>MSNAEKALGVALIGTGFMGKCHAMAWRNVATAFGGLPPRLEVLADMPADKAHSLASSFGFARGTADWREAVSDPAVDVVSITTPNGLHREMAEAALAAGKHVWLEKPMALSVEDAQAMEAAARASDRRTIIGYNYTRSPAFRAAVDLIAEGAIGRPIHFRGMYDEDYMADPDLPWSWALTRKDGGLGALGDLGCHLVSVMVSLMGPVARVYAQADTVITDRPHQGGTARVENEDQAQALIRFASGTSGEFSCSRVARGYRCRLAWEVQGTEGTLRFDQERMNE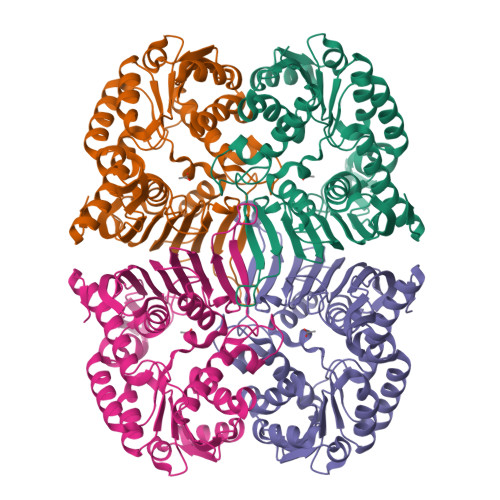LWLYQPGRPEIDGFRRILTGPAQPGFAAFCPGGGHNFGFNEQKVVEAEMLRQAIAGRGKAWPDFTDGLTIERVIHGMATSAQTGQPVNFLEHHHHHH[4x]Copper-containing nitrite reductases (CuNIRs) catalyze transformation of nitrite to nitric oxide, which has impacts on geochemical, agricultural, and medical health fields. CuNIRs typically have an ∼110 kDa homotrimeric structure, like a Reuleaux triangle. Each protomer contains one type 1 copper (T1Cu) and one type 2 copper (T2Cu) site. The Cys residue forms a peptide-bond bridge (Cys-His bridge) together with one of the His ligands at the T2Cu site to transfer the electron to the catalytic T2Cu site, which is coordinated by three His residues and an axial water molecule.

We therefore used the C135A mutant, in which the Cys residue of the Cys-His bridge is replaced with Ala. The Ala residue does not coordinate to the T1Cu atom, thereby greatly suppressing ET from T1Cu to T2Cu. Moreover, we performed the experiment at cryogenic temperature (100 K) to trap the NO2--bound state, which spontaneously decomposes during room temperature (RT) neutron data collection over a week. NX joint refinement was performed using reflections up to 1.70 Å resolution for ND and 1.30 Å resolution for XRD data. The ligand was modeled as a mixture of a major NO2- ligand (occupancy 0.7) and a minor water ligand (occupancy 0.3). The neutron-scattering length density map shows that the nitrite ligand is in the deprotonated form (NO2-) rather than in the protonated HNO2 form; thus, it does not form an H-bond with AspCAT. The shortest distance between NO2- and AspCAT is 3.2 Å, indicating that there is only a van der Waals contact. The NO2- ligand shows a κ1-O coordination manner with Cu-Onitrite distances of 1.8 and 2.7 Å. The 2mFo-DFc neutron-scattering length density map shows D atoms on the two N atoms in the imidazole ring of HisCAT, showing that HisCAT is protonated in the substrate-bound state at pD5.9. In contrast, AspCAT is in the deprotonated state.

> NVIAAHKGVNQAPVPLKMERVGPHDVHIEMTAQITDIEIDKGKIYKAWTFNGQAPGPLVVVNEGDTIHFTLKNMDPVVPHSMDFHAVHASPSKDFIDVMPNKSGTFTYPANKPGVFMYHAGTKPVLQHIANGMHGVIIVKPKNGYPTDKEVDREYVLIQNEWYKYNDMNDFQNGVPSYVVFSSKALKPGDPNTNGDTFTLKEKPLLAKVGEKIRLYINNVGPNEVSSFHVVGTVFDDVYLDGNPNNHLQGMQTVMLPASGGAVVEFTVTRPGTYPIVTHQFNHAQKGAVAMLKVTETGED>[3x]XP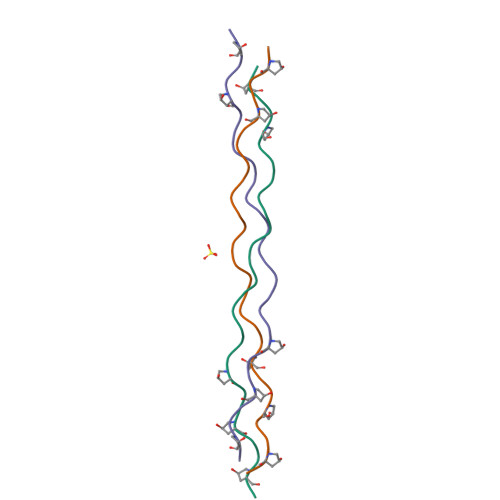PGPPGQRGREGPMGPRGPPGPPGPPGX> GAMANKAPS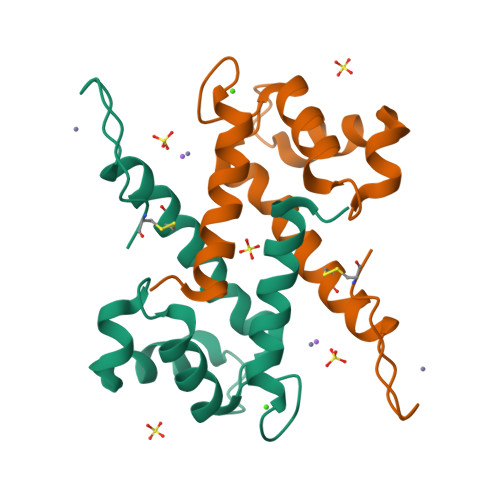QMERSITTIIDTFHQYSRKEGHPDTLSKKEFRQMVEAQLATFMKKEKRNEALINDIMEDLDTNQDNQLSFEEAMMLMAKLIFACHEKLHENNPRGHGHSHGKGCGK> SMGEIESYCNKELGPLPTKAPTLSKNV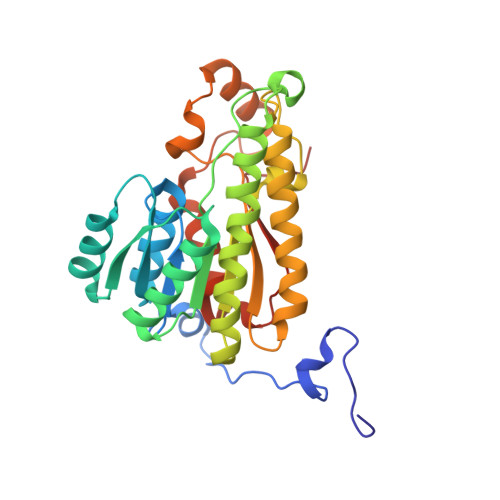LDLFSLKGKVASVTGSSGGIGWAVAEAYAQAGADVAIWYNSHPADEKAEHLQKTYGVHSKAYKCNISDPKSVEETISQQEKDFGTIDVFVANAGVTWTQGPEIDVDNYDSWNKIISVDLNGVYYCSHNIGKIFKKNGKGSLIITSSISGKIVNIPQLQAPYNTAKAACTHLAKSLAIEWAPFARVNTISPGYIDTDITDFASKDMKAKWWQLTPLGREGLTQELVGGYLYLASNASTFTTGSDVVIDGGYTCP> MAEYLIDLTPRMAYVDRHELLRSLLTEKEFIERRQEQLNKSTTVYVGNLSFYTTEDQIWEHFSRCGHIRDLVMGLSEVTRTPCGFCFVVFESQDGAMSAVIDLHGTLLDDRVITVSWDVGCDHTRRWGRGAHGGQVVDGVRQNLDSARGGLGVLRREELGVGAAVAED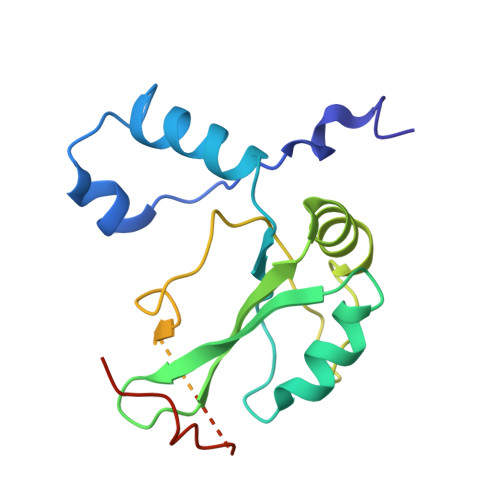QLVHYTWIPPRRVEKRGRS Glutathione transferases (GSTs; EC 2.5.1.18) are phase II detoxification enzymes that metabolize a wide range of hydrophobic toxic compounds by catalyzing the conjugation of glutathione (GSH) to the hydrophilic centre of the toxic substances. In the present study, we report the kinetic characterization and crystal structure determination of Atu3701 protein from A. tumefaciens. Sequence and structural analysis indicate that Atu3701 defines a novel GST class distinct from other previously characterized GSTs. AtuGSTH1-1 exhibits wide substrate specificity although analysis of the catalytic efficiency (kcat/Km) suggests that hydroperoxides may be its ‘natural’ substrates, indicating that the enzyme may play important role in counteracting oxidative stress conditions.

The structure of AtuGSTH1-1 exhibits the characteristic overall fold of GSTs that comprises an N-terminal thioredoxin-like domain and a C-terminal all α-helical domain. Close inspection shows that the formation of the dimer follows the ‘lock-and-key’ mode that is also found in the phi, alpha, mu and pi classes of GSTs. A molecule of Nb-GSH was found bound in the active site of AtuGSTH1-1. The glutathione portion of Nb-GSH is located in a region formed by the beginning of helices H1 and H4 and part of the β-turn between H3 and β3. In contrast to other GSTs where the H-site involves C-terminal domain residues, interactions in AtuGSTH1-1 are mainly provided by Arg187 and the long turn between strand β1 and helix H1 (residues 25–33). Analysis of the structure of AtuGSTH1-1 showed the absence of any functional side-chain (Ser, Tyr, Cys) in hydrogen bond distance with the cysteinyl moiety of the bound Nb-GSH. Indeed, the Arg34Ala mutant was inactive (kcat approximately 0.01 min−1), indicating that Arg34 may represent an important catalytic residue. In the AtuGSTH1-1/Nb-GSH complex, the conserved residues Arg34, Glu85, Ser86, Gln68 and Asn120' appear to form the proposed electron-sharing network. Arg34 in AtuGSTH1-1 occupies two alternative positions and exhibits high crystallographic temperature factors, indicating significant flexibility. In particular, in one conformation its guanidium group interacts with the γ-glutamyl carboxylate of GSH forming an electrostatic interaction, while in the second conformation with the sulfur atom of Nb-GSH (3.4 Å), the water molecules W117 and W304, and the backbone carbonyl group of bound Nb-GSH.

> MSNIETVPASIEMKPNPTITVFERSPDGGRGLARDMPVRWALEEVGQPYHVRRLSFEAMKEASHLAYQPFGQIPSYEQGDLILFESGAIVMHIAQHHSGLLPEDQLRRARTVAWMFAALNTIEPSILNFTTVWLFERNEPWHEARLARTKEQLLKRLDELSAWLGDREWLEGSFSAADILMICVLRRLESSGILKDYGNLLAYVERGKARPAFKRAFDAQLAVFTAASKN Here, we present the cryo-EM structure of CalA3, a chain release PKS module without an ACP domain, and its structures with amidation or hydrolysis products. The domain organization reveals a unique “∞”-shaped dimeric architecture with five connected domains. The catalytic region tightly contacts the structural region, resulting in two stabilized chambers with nearly perfect symmetry while the N-terminal docking domain is flexible. The ~360 kDa megaenzyme uses only the KS domain to catalyze one C–N bond formation (or hydrolysis) and subsequently release the polyketide chain.

The substrates (SNAC-N1 and 3-HAA, discussed later) were added into the CalA3 solution for cryo-EM sample preparation. The cryo-EM maps of CalA3 at overall resolutions of 3.38 Å and 4.55 Å were ultimately reconstructed. Although the two substrates were not observed, the resolution of the maps enabled us to reliably assign the individual domains, dissect their linker junctions, and build atomic models of CalA3. The dimeric CalA3 adopts an “∞” shape in both front and back views, with dimensions of approximately 193 × 87 × 116 Å3. CalA3 is composed of two regions: the lower condensing (KS-AT) and the upper modifying (DH-ψKR/KR) regions. Since CalA3 KS does not catalyze Claisen condensation and DH-KR is likely inactive (discussed later), it is more reasonable here to describe them as catalytic (KS-AT) and structural (DH-ψKR/KR) regions. Intriguingly, distinct from the catalytic and structural regions being loosely connected, which was observed in mFAS, LovB, and MAS-like PKS, the structural region of CalA3 substantially contacts the catalytic region, resulting in interfaces that account for nearly 50% of the total buried surface area, with approximately 1421 Å2 on each side, mainly through hydrogen bonding and ionic interactions between the LinkerDH-KR/ψKR and LD-AT domains of opposite chains. We observed two different rotational locations of DD in CalA3. Similarly, the substrate tunnel of the KS monomer traverses through with an open end; however, the two-sided tunnel of the KS dimer is intercepted by the F148 residue pair that forms the aromatic-aromatic interaction with a 4.5 Å distance. The active site residues containing C197, H332, and H372 are conserved, but C197 rotates approximately 143° relative to the same positioned Cys residues in the homologs.

>MPDEEKLQKYLRKVTAELQQARRRLAAAESQSQEPIAVLGIGCRFPGGVRSPEDLWDLVDSGGDAVGGLPAGRGWQAGSALDGVNAGFIHGVEEFDPYFFGLDPVEAAAMDPQQRLLLETTWEAFERAGIDPVAARGSRTAVYAGVQFGGYPLLMREAPPPQVLDHLGLGNSVGAASGRLAYQFGLLGGAVTVDTQCTSSIVALHLAVKALRNGECALALAGGACVMSLPTVLMDFHRRSLLAPDGRSKSFAAAADGVSLAEGAGMLLLERLSDARRNGHPVMAVIRGTAINQDGATNGIISPSGRAQERVIRAALADGRVTADSVDAVEGHGVGATLGDGVEVTSLLSTYGQERPAGRPLLLGSVKSNIGHTQTVGAVAGIVKLVMALRNERLPRTVHVDGPTPHADWSSGTVRLLTEPEPWRRGERVRRAGLTCLTLSGTNGHLILEEPPADEPAARPANPERTVPLVLSAKSPTALREQAERLRATITAAEPVDVGHSLHTTRSSFRHRAVVLGTGREELAAGLDALAGDRTADGLVRGVARAQGQTALLFGGAGDGTSGDRPADAEGPRTARGLYEAFPAFAEALDEVTEHLAGLLGPEVRAAVREPGPACAEPTVVGQAVAFALNTALHRLLTAFAVRPDATLGHGAGEVAAAYAAGALSLADGAALVTALGRITERVATGPGASVWVRATEDEVRAALSGSQEQVGAAVAAVDEPGTTVVSGDAGAVARVAAHWRAHGRATGAPRPARLLLSPDDEQAALAELRAIVAGLAFREPEVPLLSTVTGQPVEPAELRSAEHWLDHLRGPTRFLDGVRRLRTDGVTRLVGLDLSGDLTGPAGRSAAGFGEPGRPLLLASVPGGGRPPGQALLSALGELHTDGVAIDWSQAFEGRGARRVDLPTYPYQKVRCWLVPPEPQVSVVAAPPHPLLGTALDLVDATGQSFTQQLTPGQVAGVFGQQLYGTPVLPAGARLEWLLAAARHGSPDSAWTLTGIRLPGTVSAASGTPVALQTSREDSGDGHRVRAFVKGPGTGGGRWAERGGATVVPAVTRPAPDRVDPESLPEGLAELDVAEVYRRLWRQGSDYAEPLRVLRRVWLGGDEAVALVGTADVPTGPSGWSRWAAVLEAAVQLAALSGSGPRTPVSVDRLEVSGPPSEVVWLRVRHGADGAADAVVLSGEGVRLAAVQGLRLRPMAGREPAGLAEAPLERHEVVWHALAEDGRPGAIGGGTGSWLVFSDDPERAAAWCDELALFGVPAVALAGEDAEGRDGTETVPVGTGDPDVVGKTFAELRERGVTVAGLLVHDAGDAREPASGADDPLDAACRRGGRTLALVRGFLQEYAEQTPRIVLCSAGAAAGLAGGPPHPAQAPLTALFTSLVWEHPELPCAQVDLDPAEDPPTVVSLLGQVMRLPGAGRLAVRGGRWFEARLERRPAPADRGERLALRPDATYLVAGGDTRHAAAALEWLAARGARSVVLAGAESERGDLAGARTTGHAGIERLEHVAVDLSSAADVARLAELCADGRPPLRGVLLLPQPVAGGGLDELDGARFGAELAGALRGPVELTRRFTDVGLTGGTDFFVLSTSVVSLPGRAGTVVGSAADAFLTALARHHRQAGLPVVAAAWGPWLESVDESDEAPAVAFAEAGVYPAPGGEMLDALLPLPAAGEADGSGEAGLARVDWDRYLTAGHRPLPYTVLETRASYDEEKAPGFGQNRMKGARKKKGAAALEHHHHHH[2x]>NMAGMNDKASMNDKASMTVKINESLPQGNGKALGTVTVTETAYGLLFTPHLTGLA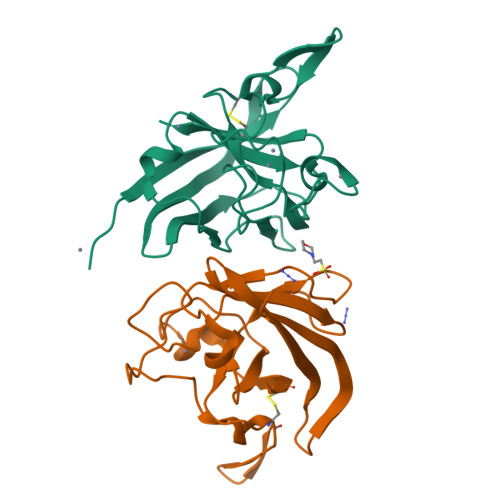PGIHGFHLHEKPSCAPGMKDGKAVPALAAGGHLDPNKTGVHLGPYNDKGHLGDLPGLVVNADGTATYPVLAPRLKSLSEVKQHALMIHAGGDNYSDHPMPLGGGGARMACGVIE[2x]> EV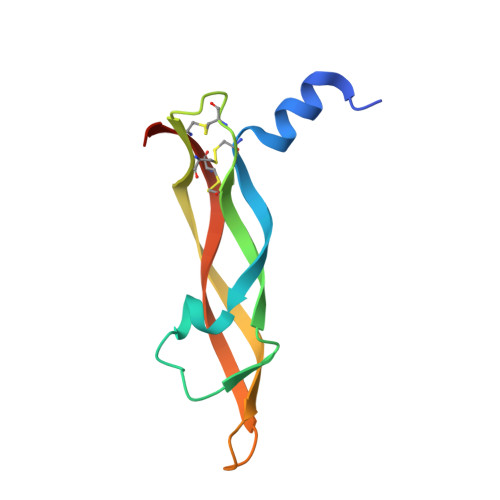EVVPFQEVWGRSYCRALERLVDVVSEYPSEVEHMFSPSCVSLLRCTGCCGDENLHCVPVETANVTMQLLKIRSGDRPSYVELTFSQHVRCECRPLREKM> ESSVTLFGIVDTNVAYVNKDAAGDSRYGLGTSGASTSRLGLRGTEDLGGGLKAGFWLEGEIFGDDGNASGFNFKRRSTVSLSGNFGEVRLGRDLVPTSQKLTSYDLFSATGIGPFMGFRNWAAGQGADDNGIRANNLISYYTPNFGGFNAGFGYAFDEKQTIGTADSVGRYIGGYVAYDNGPLSASLGLAQQKTAVGGLATDRDEITLGASYNFGVAKLSGLLQQTKFKRDIGGDIKTNSYMLGASAPVGGVGEVKLQYALYDQKAIDSKAHQITLGYVHNLSKRTALYGNLAFLKNKDASTLGLQAKGVYAGGVQAGESQTGVQVGI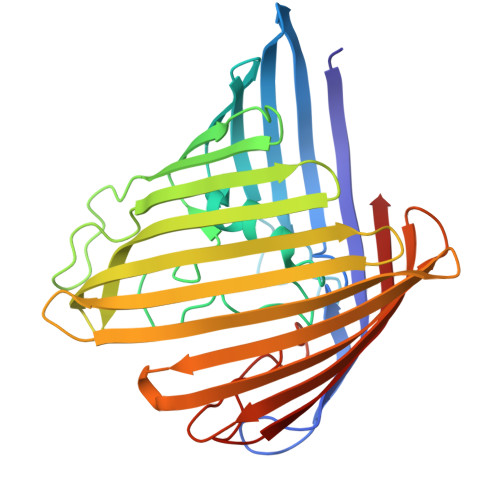RHAF> VEKLTADAELQRLKNERHEEAELERLLSEY;> LSECKTGNGKNYRGTMSKTKNGITCQKWSSTSPHRPRFSPATHPSEGLEENYCRNPDNDPQGPWCYTTDPEKRYDYCDILECEEECMHCSGENYDGKISKTMSGLECQAWDSQSPHAHGYIPSKFPNKNLKKNYCRNPDRELRPWCFTTDPNKRWELCDIPRCTTPPPSSGPTYQCLKGTGENYRGNVAVTVS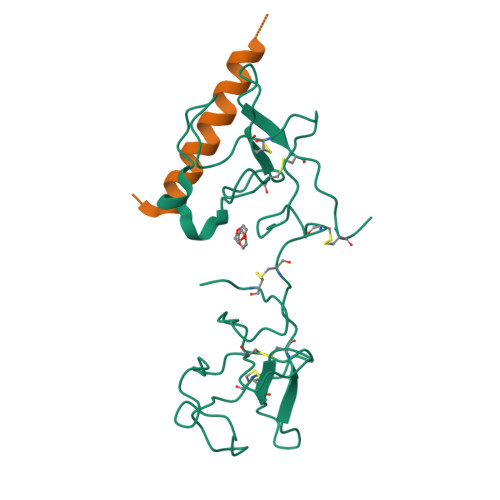GHTCQHWSAQTPHTHERTPENFPCKNLDENYCRNPDGKRAP>[3x]MSLQRIVRVSLEHPTSAVCVAGVETLVDIYGSVPEGTEMFEVYGTPGVDIYISPNMERGRERADTRRWRFDATLEIIVVMNSPSNDLND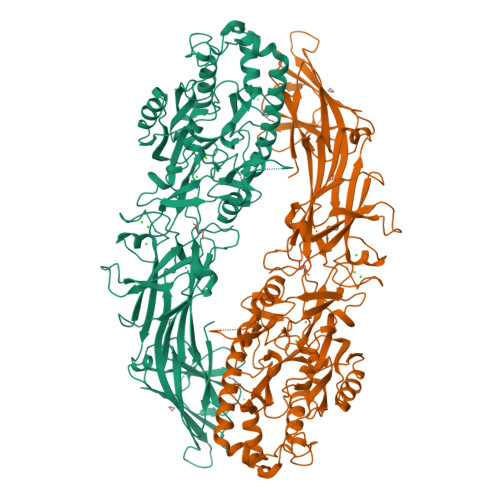SHVQISYHSSHEPLPLAYAVLYLTCVDISLDCDLNCEGRQDRNFVDKRQWVWGPSGYGGILLVNCDRDDPSCDVQDNCDQHVHCLQDLEDMSVMVLRTQGPAALFDDHKLVLHTSSYDAKRAQVFHICGPEDVCEAYRHVLGQDKVSYEVPRLHGDEERFFVEGLSFPDAGFTGLISFHVTLLDDSNEDFSASPIFTDTVVFRVAPWIMTPSTLPPLEVYVCRVRNNTCFVDAVAELARKAGCKLTICPQAENRNDRWIQDEMELGYVQAPHKTLPVVFDSPRNGELQDFPYKRILGPDFGYVTREPRDRSVSGLDSFGNLEVSPPVVANGKEYPLGRILIGGNLPGSSGRRVTQVVRDFLHAQKVQPPVELFVDWLAVGHVDEFLSFVPAPDGKGFRMLLASPGACFKLFQEKQKCGHGRALLFQGVVDDEQVKTISINQVLSNKDLINYNKFVQSCIDWNREVLKRELGLAECDIIDIPQLFKTERKKATAFFPDLVNMLVLGKHLGIPKPFGPIINGCCCLEEKVRSLLEPLGLHCTFIDDFTPYHMLHGEVHCGTNVCRKPFSFKWWNMVP> DTALERQIASASRSVEEARRLAYHDPIRVGALVEQISVLADLRQKEGDFRKAESLYREALFRAQELRKQDPDLLTGIYSLLAHLYDRWGRMDKAAEFYELALKISAENGLEESDKVATIKNNLAMIFKQLRKFERAEGYYCEALETFQRLDGEQSARVASVYNN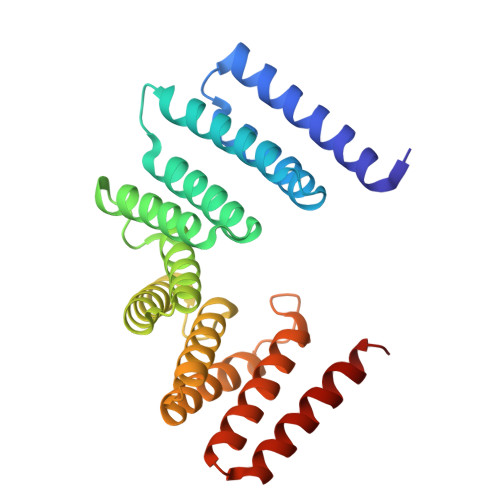LGVLYYSHMDVDRAQVMHERALAIRQNLHEGQMDPADLSQTFINLGAVYKAAGDFQKAEACVDRAKRIRAAMNG>GSHMGEGVQLTAAQELMIQQLVAAQLQCNKRSFSDQPKVTPWPLGADPASGSASQQRFAHFTELAIISVQEIVDFAKQVPGFLQLGREDQIALLKASTIEIMLLETARRYNHETECITFLKDFTYSKDDFHRAGLQVEFINPIFEFSRAMRRLGLDDAEYALLIAINIFSADRPNVQEPGRVEALQQPYVEALLSYT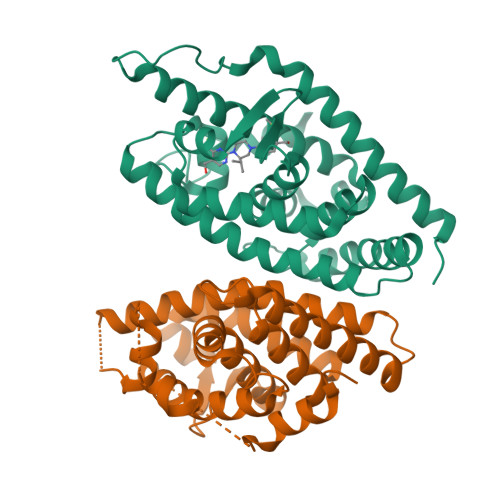RIKRPQDQLRFPRMLMKLVSLRTLSSVHSEQVFALRLQDKKLPPLLSEIWDVHEGSGSGSHKILHRLLQDSSS[2x];>[2x]MGAPEEMPVDRILEAELAVEQKSDQGVEGPGGTGGSGSSPNDPVTNICQAADKQLFTLVEWAKRIPHFSSLPLDDQVILLRAGWNELLIASFSHRSIDVRDGILLATGLHVHRNSAHSAGVGAIFDRVLTELVSKMRDMRMDKTELGCLRAIILFNPDAKGLSNPSEVEVLREKVYASLETYCKQKYPEQQGRFAKLLLRLPALRSIGLKCLEHLFFFKLIGDTPIDTFLMEMLEAGSGSGSHKILHRLLQDSSS>[2x]GSSGALLFHGKIPYVVEME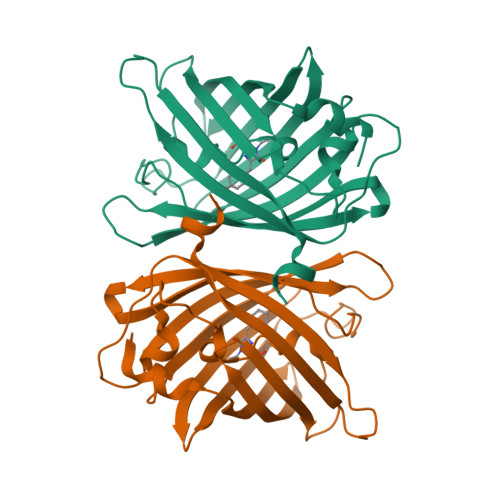GNVDGHTFSIRGKGYGDASVGKVDAQFICTTGDVPVPWSTLVTTLTYGAQCFAKYGPELKDFYKSCMPDGYVQERTITFEGDGNFKTRAEVTFENGSVYNRVKLNGQGFKKDGHVLGKNLEFNFTPHCLYIWGDQANHGLKSAFKICHEITGSKGDFIVADHTQMNTPIGGGPVHVPEYHHMSYHVKLSKDVTDHRDNMSLKETVRAVDCRKTYDFDAGSGDTSLIS>[2x]KRGIDLKVQPQEPLVLKDVENTDWRLLRGDTDVRVERKDPN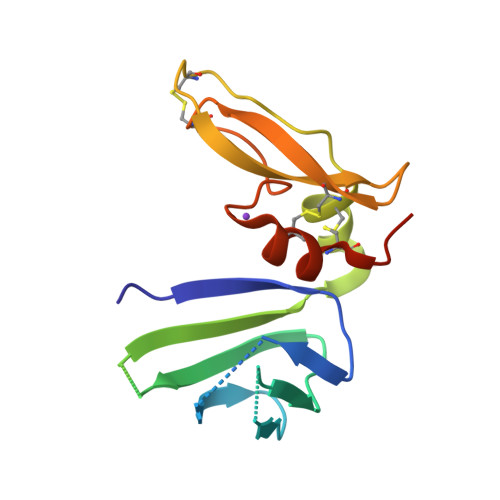QVELWGLKEGTYLFQLTVTSSDHPEDTANVTVTVLSTKQTEDYCLASNKVGRCRGSFPRWYYDPTEQICKSFVYGGCLGNKNNYLREEECILACRGVDHHHHHH> YFGKLESKLSVIRNLNDQVLFIDQGNRPLFEDMTDSDCRDNAPRTIFIISMYKDSQPRGMAVTISVKCEKISTLSCENKIISFKEMNPPDNIKDTKSDIIFFQRSVPGHDNKMQFESSSYEGYFLACEKERDLFKLILKKEDELGDRSIMFTVQNED;> GPESCTSRPHITVVEGEPFYLKHCSCSLAHEIETTTKSWYKSSGSQEHVELNPRSSSRIALHDCVLEFWPVELNDTGSYFFQMKNYTQKWKLNVIRRNKHSCFTERQVTSKIVEVKKFFQITCENSYYQTLVNSTSLYKNCKKLLLENNKNPTIKKNAEFEDQGYYSCVHFLHHNGKLFNITKTFNITIVEDRSNIVPVLLGPKLNHVAVELGKNVRLNCSALLNEEDVIYWMFGEENGSDPNIHEEKEMRIMTPEGKWHASKVLRIENIGESNLNVLYNCTVASTGGTDTKSFILVRKADMADIPGHVFTR;> GPERIKGFNISGCSTKKLLWTYSTRSEEEFVLFCDLPEPQKSHFCHRNRLSPKQVPEHLPFMGSNDLSDVQWYQQPSNGDPLEDIRKSYPHIIQDKCTLHFLTPGVNNSGSYICRPKMIKSPYDVACCVKMILEVKPQTNASCEYSASHKQDLLLGSTGSISCPSLSCQSDAQSPAVTWYKNGKLLSVERSNRIVVDEVYDYHQGTYVCDYTQSDTVSSWTVRAVVQVRTIVGDTKLKPDILDPVEDTLEVELGKPLTISCKARFGFERVFNPVIKWYIKDSDLEWEVSVPEAKSIKSTLKDEIIERNIILEKVTQRDLRRKFVCFVQNSIGNTTQSVQLKEKR

Interleukin (IL)-18 belongs to the IL-1 superfamily and was first discovered as an interferon gamma (IFN-γ)-inducing factor in sera from mice with hepatitis stimulated with Propionibacterium acnes and lipopolysaccharide1. This proinflammatory cytokine is secreted by various types of cells and strongly augments IFN-γ production in type-1 helper T (Th1) cells and natural killer (NK) cells following activation of NK-cell cytotoxicity; thus, it plays a critical role in inflammation and the host defense against microbes. IL-18/IL-18Rα/IL-18Rβ ternary complex formation juxtaposes the intracellular Toll-Interleukin-1 receptor domains of IL-18Rα and IL-18Rβ, to which the adaptor molecule myeloid differentiation factor 88 (MyD88) is recruited presumably with the aid of TRAM6. We determined the crystal structures of IL-18, the IL-18/IL-18Rα binary complex and the IL-18/IL-18Rα/IL-18Rβ signalling ternary complex at the resolutions 2.33, 3.10 and 3.10 Å, respectively.

The IL-18/IL-18Rα/IL-18Rβ signalling ternary complex is formed by IL-18Rβ binding with the lateral portion of the binary complex. On ternary complex formation, the IL-18/IL-18Rα binary complex structure essentially does not change; the root mean square deviations (RMSD) for the backbone Cα atoms are 0.41–0.90 Å compared with the asymmetric unit (ASU) molecules. D2 and D3 of IL-18Rβ are close to each other and directly associated with IL-18/IL-18Rα, while D1 does not contribute to ternary complex formation. The IL-18Rβ-D2 convex surface with the key Tyr212Rβ aromatic residue fits into the concave surface jointly formed by IL-18 and IL-18Rα-D2 with a 613 Å2 buried surface area, which is shallower than that in the IL-1β complexes. The concave surface area is divided into Site III on IL-18 (354 Å2) and part of IL-18Rα-D2 (259 Å2). Site III of IL-18 comprises the prominent β8-β9 hairpin and β11-α2 loop, where the aromatic ring of His109IL-18 forms π-π stacking with Tyr212Rβ at a 3.4 Å distance, which is surrounded and stabilized by multiple hydrogen bonds. In addition to these interactions, IL-18Rβ-D3 extensively contacts IL-18Rα-D3 with the buried area ~550 Å2, to which both electrostatic and hydrophobic interactions contribute. Notably, the NAG-NAG extended from the IL-18Rα-D3 Asn236Rα and points to the receptor C-terminus in the binary complex; however, in the ternary complex, the NAG-NAG chain changes direction and points to IL-18Rβ-D3 within the distance possibly to form electrostatic interaction with Val257Rβ and Asp259Rβ. As a result, despite the same ‘left’ binding mode, the spatial arrangements of the subdomains in the IL-18/IL-18Rα/IL-18Rβ ternary complex differ somewhat from IL-1β/IL-1RI/IL-1RAcP with Cα atom RMSD values of 6.64–6.73 Å. Our data show that IL-18Rβ-Y212A did not bind the binary complex, which is consistent with the structure, wherein substantial π-π stacking were observed between Tyr212Rβ and His109IL-18.>[2x]MVSIRRSFEAYVDDMNIITVLIPAEQKEIMTPPFRLETEITDFPLAVREEYSLEAKYKYVCVSDHPVTFGKIHCVRASSGHKTDLQIGAVIRTAAFDDEFYYDGELGAVYTADHTVFKVWAPAATSAAVKLS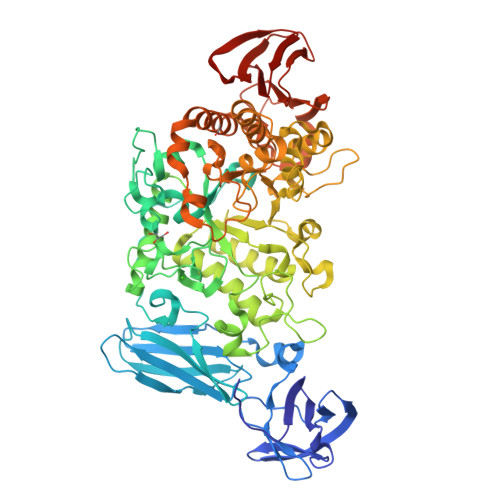HPNKSGRTFQMTRLEKGVYAVTVTGDLHGYEYLFCICNNSEWMETVDQYAKAVTVNGEKGVVLRPDQMKWTAPLKPFSHPVDAVIYETHLRDFSIHENSGMINKGKYLALTETDTQTANGSSSGLAYVKELGVTHVELLPVNDFAGVDEEKPLDAYNWGYNPLHFFAPEGSYASNPHDPQTRKTELKQMINTLHQHGLRVILDVVFNHVYKRENSPFEKTVPGYFFRHDECGKPSNGTGVGNDIASERRMARKFIADCVVYWLEEYNVDGFRFDLLGILDIDTVLYMKEKATKAKPGILLFGEGWDLATPLPHEQKAALANAPRMPGIGFFNDMFRDAVKGNTFHLKATGFALGNGESAQAVMHGIAGSSGWKALAPIVPEPSQSINYVESHDNHTFWDKMSFALPQENDSRKRSRQRLAVAIILLAQGVPFIHSGQEFFRTKQGVENSYQSSDSINQLDWDRRETFKEDVHYIRRLISLRKAHPAFRLRSAADIQRHLECLTLKEHLIAYRLYDLDEVDEWKDIIVIHHASPDSVEWRLPNDIPYRLLCDPSGFQEDPTEIKKTVAVNGIGTVILYLASDLKSFA> GSMRHILERPDPTDVFQNKANVCWAKALVPVLKTAGIDMTTEQWNTVDYFETDKAHSAEIVLNQLCVRFFGLDLDSGLFSAPTVPLSIRNNHWDNSPSPNMYGLNKEVVRQLSRRYPQLPRAVATGRVYDMNTGTLRNYDPRINLVPVNRRLPHALVLHHNEHPQSDFSSFVSKLKGRTVLVVGEK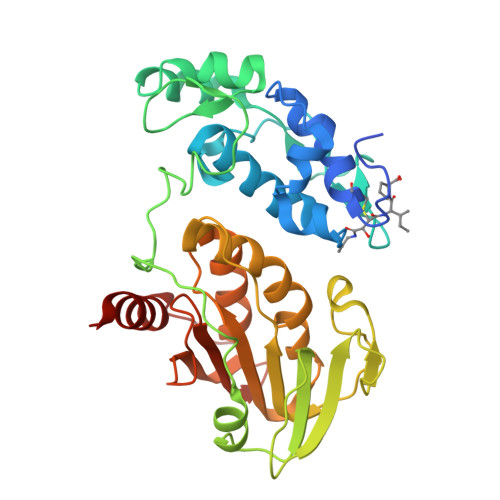LSVPGKMVDWLSDRPEATFRARLDLGIPGDVPKYDIIFVNVRTPYKYHHYQQCEDHAIKLSMLTKKACLHLNPGGTCVSIGYGYADRASESIIGAIARQFKFSRVCKPKSSLEETEVLFVFIGYDRKARTHNPYKLSSTLTNIYTGSRLHEA>[2x]MAPSRKFFVGGNWKMNGRKQSLGELIGTLNAAKVPADTEVVCAPPTAYIDFARQKLDPKIAVAAQNCYKVTNGAFTGEISPGMIKDCGATWVVLGHSERRHVFGESDELIGQKVAHALAEGLGVIACIGEKLDEREAGITEKVVFEQTKVIADNVKDWSKVVLAYEPVWAIGTGKTATPQPAQEVHEKLRGWLKSNVSDAVAQSTRIIYGGSVTGATCKELASQPDVDGFLVGGASLKPEFVDIINAKQ

Triosephosphate isomerase (TPI) deficiency (TPI Df) is an untreatable glycolytic enzymopathy that results in hemolytic anemia, progressive muscular impairment and irreversible brain damage. TPI is a homodimer with each monomer adopting the (βα)8 TIM barrel fold. Access to the catalytic site is restricted by the catalytic lid which is formed by loop 6. Transitions between the open and closed state of the catalytic lid are coordinated with changes in the positions of prominent residues within the active site including E165, K13, H95 and S96.

Comparing the structures of wild-type TPI and TPIQ181P, we found that they are highly similar overall as expected with an all atom root mean square deviation (r.m.s.d.) of 0.24 Å, demonstrating that the overall fold of TPI was not disturbed by the mutation. The first is within the catalytic lid, which we found to be disordered within the TPIQ181P structure. We observed this in both subunits of the dimer; however, the affected regions were not identical, with residues 170-177 being disordered in subunit A, whereas residues 172-179 were disordered in subunit B. The electron density was clearer for the P181 residue in subunit A (inset), and thus we use this subunit in our figures and description unless otherwise noted. A proline at position 181 not only disrupts these interactions but also introduces a kink in the main chain, which prevents residues 177-181 from adopting the helical conformation observed in wild-type TPI structures. Residues 177-181 are observed in a helical conformation in both the open and closed orientation of the catalytic lid, demonstrating that the defect observed is not merely altering the equilibrium between the open and closed states, but is instead grossly affecting the C-terminal hinge and catalytic lid. We crystallized TPIQ181P in the presence of bromide, which we have shown previously to localize in the active site along with a phosphate abstracted from solution. In our TPIQ181P structure, however, we observed only partial occupancy for bromide ions, and no phosphates were observed. Further, we found that residues E165 and S96 adopted the open conformation.> MSLRRGIYHIENAGVPSAIDLKDGSSSDGTPIVGWQFTPDTINWHQLWLAEPIPNVADTFTLC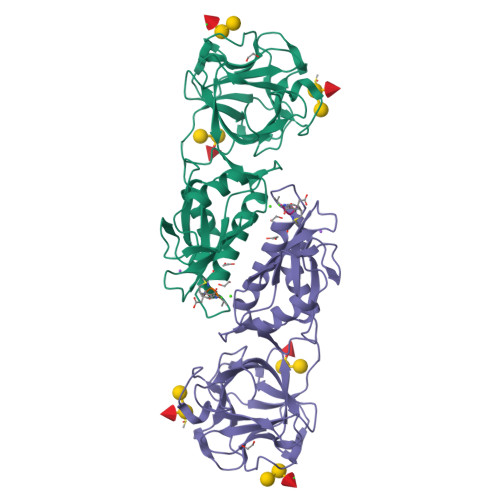NLFSGTYMDLYNGSSEAGTAVNGWQGTAFTTNPHQLWTIKKSSDGTSYKIQNYGSKTFVDLVNGDSSDGAKIAGWTGTWDEGNPHQKWYFNRMSVSSAEAQAAIARNPHIHGTYRGYILDGEYLVLPNATFTQIWKDSGLPGSKWREQIYDCDDFAIAMKAAVGKWGADSWKANGFAIFCGVMLGVNKAGDAAHAYNFTLTKDHADIVFFEPQNGGYLNDIGYDSYMAFY> SHMSSTSPNLQKAIDLASKAAQEDKAGNYEEALQLYQHAVQYFLHVVKYEAQGDKAKQSIRAKCTEYLDRAEKLKEYLKNKEKKAQKPVKEGQPSPADEKGNDSDGEGESDDPEKKKLQNQLQGAIVIERPNVKWSCVAGLEGAKEALKEAVILPIKFPHLFTGKRTPWRGILLFGPPGTGKSYLAKAVATEANNSTFFSISSSDLVSKWLGES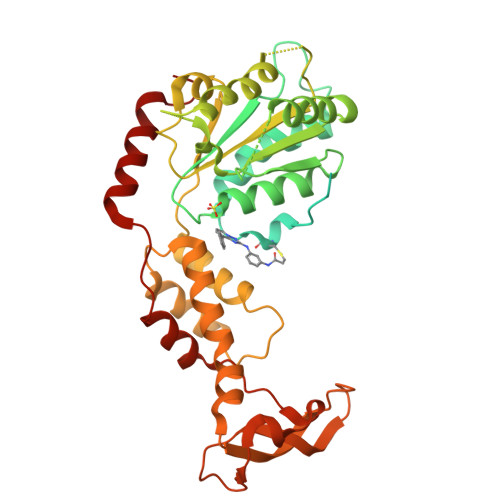EKLVKNLFQLARENKPSIIFIDEIDSLCGSRSENESEAARRIKTEFLVQMQGVGVDNDGILVLGATNIPWVLDSAIRRRFEKRIYIPLPEPHARAAMFKLHLGTTQNSLTEADFRELGRKTDGYSGADISIIVRDALMQPVRKVQSATHFKKVRGPSRADPNHLVDDLLTPCSPGDPGAIEMTWMDVPGDKLLEPVVSMSDMLRSLSNTKPTVNEHDLLKLKKFTEDFGQEG>AMAGVYTYENEFTSDIPAPKLFKAFVLDADNLIPKIAPQAVKCAEILEGDGGPGTIKKITFGEGSHYGYVKHKIHSIDKVNHTYSYSLIEGDALSENIEKIDYETKLVSAPHGGTIIKTTSKYHTKGDVEIKEEHVKAGKEKAAHLFKLIEGYLKDHPSEYN[6x]

Fra a proteins are members of the pathogenesis-related 10 family and are required for the normal accumulation of flavonoids and the development of color in strawberry fruits. PR-10 proteins belong to the START superfamily. These proteins adopt a helix-grip fold with an internal cavity capable of binding hydrophobic ligands. The data presented here demonstrates that Fra a proteins bind natural flavonoids, providing for the first time mechanistic insight on the function of these proteins in the control of flavonoid biosynthesis.

The refined model contains six molecules of Fra a 1E in the asymmetric unit. None of these molecules contained catechin inside the cavity. However, a molecule of catechin was found at the surface of molecule F between two Fra a 1E subunits in adjacent asymmetric units. The nature of the interaction suggests that this catechin molecule has been captured as a consequence of the crystallization process. As expected, the six molecules in crystal form B show a very similar structure, which is also similar to that of crystal form A. However, a high degree of conformational variation is observed in the loop regions L3, L5, and L7. In particular loop L5, shows a distinct conformation in every of the six molecules found in the asymmetric unit. These conformations range from a “closed” conformation, represented by molecule C, in which loop L5 is folded over the central cavity of the protein and approaches the C-terminal α-helix (colored green in Fig. 3b), to an “open” conformation represented by molecule F, in which loop L5 is at a maximal distance from the C-terminal α-helix (colored orange in Fig. 3b). Molecule C in crystal form B of Fra a 1E, is the one that more closely resembles the Fra a 3 catechin complex with loop L5 approaching helix α3. However, in this case, loop L3 adopts an open conformation, and the bend in helix α3 is not present.(2E)-3-{5-[(2,4-diaminopyrimidin-5-yl)methyl]-2,3-dimethoxyphenyl}-1-[(1S)-1-(4-methylphenyl)phthalazin-2(1H)-yl]prop-2-en-1-one | 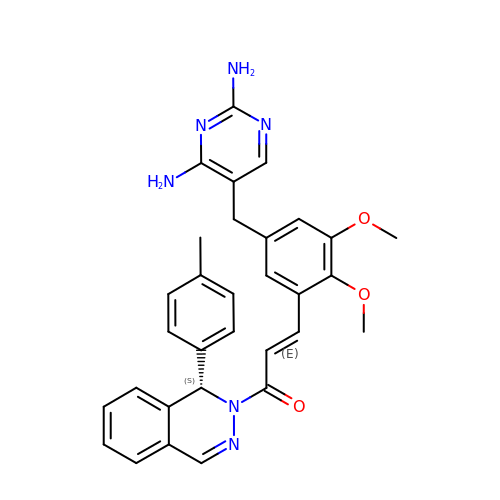C31 H30 N6 O3 | YQJQZCMRSICFNE-DTQJJDMLSA-N> MAFARGGLAQTASQTTSSPVRVGLSVDASALGHTIPPDYTGLSYEQAQMANPNYFSGANTQLAGFLRTLGRQGVLRIGGNTSEYTFWNRHAKPTAADEHLAAGPDKGHHAAAREVITPEAVNNLSEFLDKTGWKLIYGLNLGKGTPENAADEAAYVMETIGADRLLAFQLGNEPDLFYRNGIRPASYDFAAYAGDWQRFFTAIRKRVPNAPFAGPDTAYNTKWLVPFADKFKHDVKFI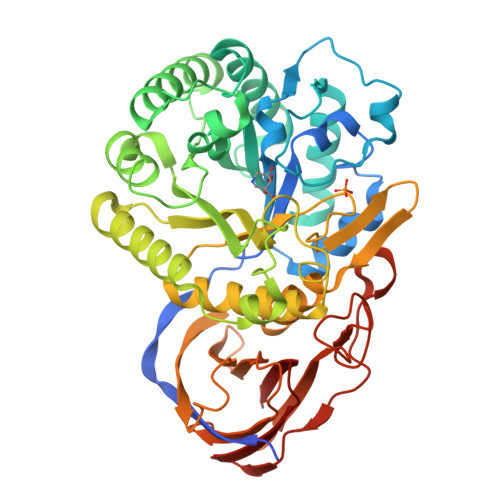SSHYYAEGPPTDPSMTIERLMKPNPRLLGETAGLKQVEADTGLPFRLTETNSCYQGGKQGVSDTFAAALWAGDLMYQQAAAGSTGINFHGGGYGWYTPVAGTPEDGFIARPEYYGMLLFAQAGAGQLLGAKLTDNSAAPLLTAYALRGTDGRTRIALFNKNLDADVEVAISGVASPSGTVLRLEAPRADDTTDVTFGGAPVGASGSWSPLVQEYVPGHSGQFVLHMRKASGALLEFA(6S)-1-[3,5-bis(trifluoromethyl)phenyl]-6-{(5M)-5-(3,5-dimethyl-1,2-oxazol-4-yl)-1-[(1s,4R)-4-methoxycyclohexyl]-1H-benzimidazol-2-yl}piperidin-2-one 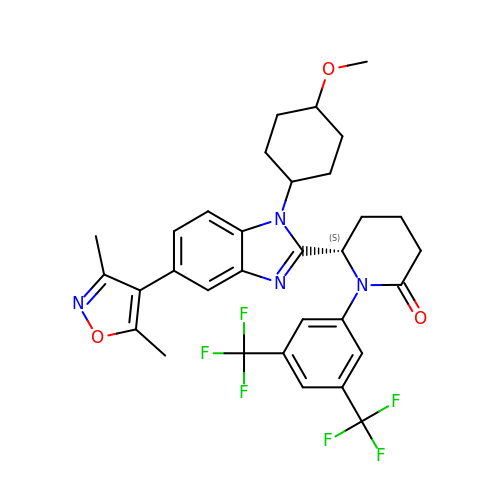| C32 H32 F6 N4 O3 | YULWSGWLJURFFP-LLGBQNBKSA-N> MAGERFPADFVWGAATAAYQIEGAVREDGRGVSIWDTFSHTPGKIADGTTGDVACDSYHRYGEDIGLLNALGMNAYRFSIAWPRIVPLGAGPINQAGLDHYSRMVDALLGAGLQPFVTLYHWDLPQPLEDRLGWGSRATATVFAEYADIVVRQLGDRVTHWATLNEPWCSAMLGYYLGVHAPGHTDLKRGLEASHNLLLGHGLAVQAMRAAAPQPLQIGIVLQLTPTYPASDSPEDVAAARRFDGFVNRWFLDPLAGRGYPQDMLDYYGAAAPQANPEDLTQIAAPLDWLGVNYYERMRAVDAPDASLPQAQRLDDPDLPHTADREVYPEGLYDILLRLHNDYPFRPLYITENGCALHDEIAEDGGIHDGQRQAFFEAHLAQLQRALAAGVPLK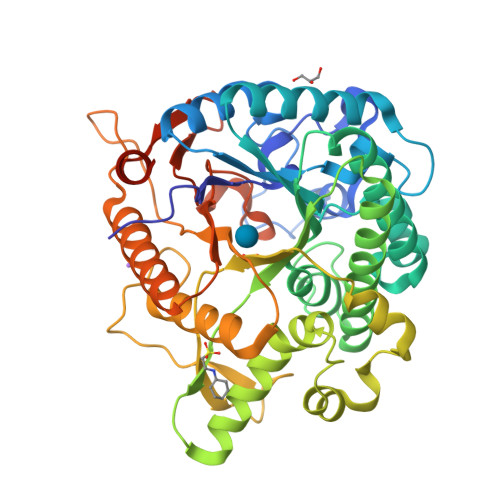GYFAWSLLDNFEWAMGLSMRYGICYTNFETLERRIKDSGYWLRDFIAGQRGKLAALEHHHHHH>[2x]ATRSPGVVISDDEPGYDLDLFCIPNHYAEDLERVFIPHGLIMDRTERLARDVMKEMGGHHIVALCVLKGGYKFFADLLDYIKALNRNSDRSIPMTVDFIRLKSYCNDQSTGDIKV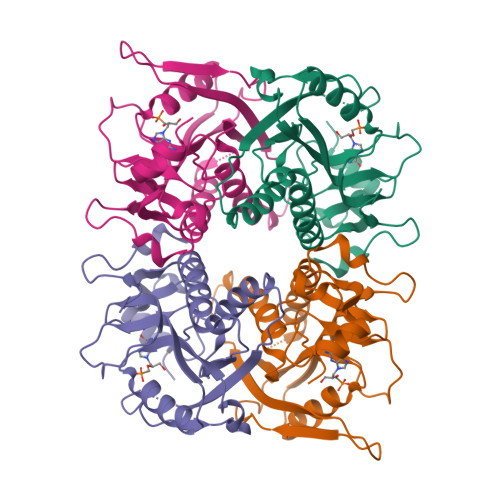IGGDDLSTLTGKNVLIVEDIIDTGKTMQTLLSLVRQYNPKMVKVASLLVKRTPRSVGYKPDFVGFEIPDKFVVGYALDYNEYFRDLNHVCVISETGKAKYKA>AGMSEAPRAETFVFLDLEATGLPSVEPEIAELSLFAVHRSSLENPEHDESGALVLPRVLDKLTLCMCPERPFTAKASEITGLSSEGLARCRKAGFDGAVVRTLQAFLSRQAGPICLVAHNGFDYDFPLLCAELRRLGARLPRDTVCLDTLPALRGLDRAHSHGTRARGRQGYSLGSLFHRYFRAEPSAAHSAEGDVHTLLLIF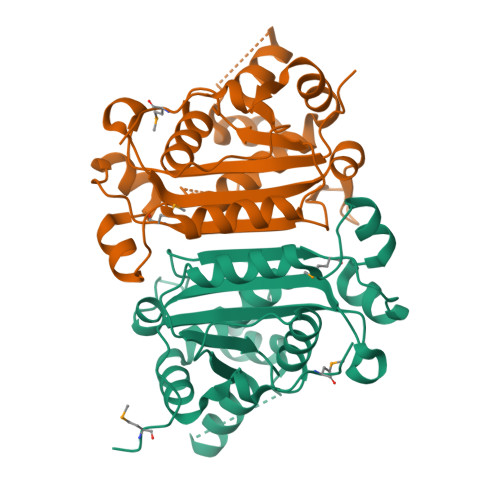LHRAAELLAWADEQARGWAHIEPMYLPPDDPSLEA[2x]> MGEPAKIYINLGVQAPGPFGGGTPEEVAATLDRVKAAAPGIGIIVDLDEGSGVHRDSDHVRLYPEGAGRYTLAEEQAIVDHAKALGAEICYHLNLTVFLPTDPVSEEERAAAKPVWTWTGLHHCIPKEKLLETLLPQKLDELEAAFPGKLDYVYLDRLFDGRCYDLTDEEVRYVLDLIKERGLGIKIESTKYLDTILESGVKVLVDEAVSEKNFDTGKAKVLDPKLFEKYPDLITVEVLYESIETIERALAAGVRNIAIHFGGYGVVSQLDEILDGVRAITENILALASAGSGHHHHHH

Here, we present a strategy for the de novo design of a simplified scaffold of an endo-α-N-acetylgalactosaminidase active site, a glycoside hydrolase from the GH101 enzyme family. Using a combination of trRosetta hallucination, iterative cycles of deep-learning-based structure prediction, and ProteinMPNN sequence design, we designed proteins with 290 amino acids incorporating the active site while reducing the molecular weight by over 100 kDa compared to the initial endo-α-N-acetylgalactosaminidase. Of 11 tested designs, six were expressed as soluble monomers, displaying similar or increased thermostabilities compared to the natural enzyme. Despite lacking detectable enzymatic activity, the experimentally determined crystal structures of a representative design closely matched the design with a root-mean-square deviation of 1.0 Å, with most catalytically important side chains within 2.0 Å.

dEngBF4 crystallized in two different space groups, P212121 (form 1) and P61 (form 2), and the crystal structures of the protein were determined using the molecular replacement method described in Materials and Methods. Form 1 has two protein molecules, 1A and 1B, in the asymmetric unit, whereas for form 2 one protein molecule is present in the asymmetric unit, resulting in three separate structures. All three structures aligned with an RMSD of 1.0 Å or less, revealing a common (β/α)8-barrel organization with an overall fold similar to the hallucinated model. Likewise, another extended loop region including His91-Lys127 harboring the two tryptophan residues, making up the tryptophan lid in EngBF, displayed both low pLDDT confidence scores and flexibility in the molecular dynamics simulation. The movement of this loop, however, is constrained due to the formation of a disulfide bond between Cys124 and Cys163 residues, potentially contributing to the observed high thermostability in dEngBF4. While ProteinMPNN proved to be highly effective in improving the pLDDT confidence score, certain loop regions remained unrecoverable, which correlated with regions displaying poor or no electron density in the crystal structure. Enzymatic assays of the dEngBF proteins with Galβ(1–3)GalNAcα1-para-nitrophenol as a substrate showed no measurable para-nitrophenol release during the designated incubation period (data not shown).> GRILFVEDEDAVRSVAARLLRARGYEVLEAADGEEALIIAEENAGTIDLL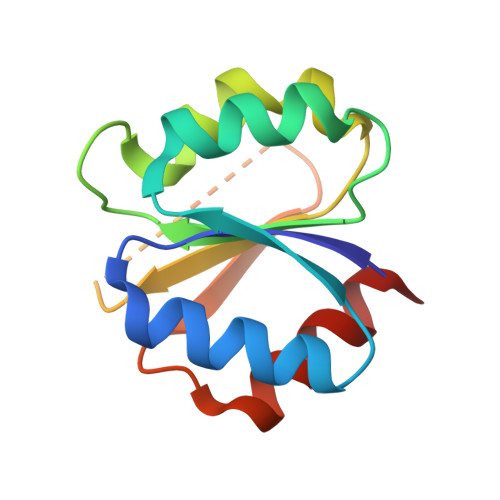ISDVIMPGIDGPTLLKKARGYLGTAPVMFISGYAEAEFSDLLEGETGVTFLPKPIDIKTLAERVKQQLQA>[4x]PKYTDKEVQQISGNLNLNIVPLFEKTLSASDAGRIGRLV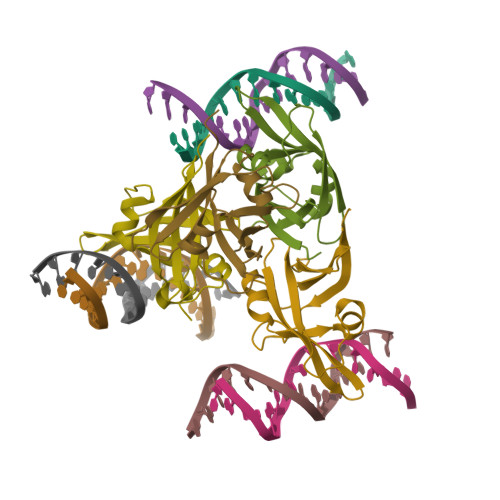LPKACAEAYFPPISQSEGIPLKIQDVRGREWTFQFRYWPNNNSRMYVLEGVTPCIQSMMLQAGDTVTFSRVDPGGKLIMGSRKAANAGD>[4x]SRPVRLMKVFVTRRIPAEGRVALARAADCEVEQWDSDEPIPAKELERGVAGAHGLLCLLSDHVDKRILDAAGANLKVISTMSVGIDHLALDEIKKRGIRVGYTPDVLTDTTAELAVSLLLTTCRRLPEAIEEVKNGGWTSWKPLW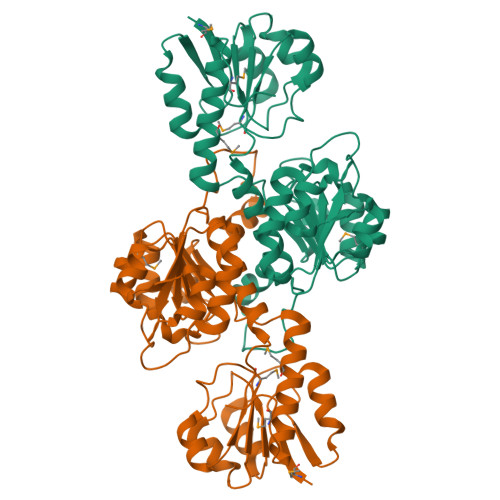LCGYGLTQSTVGIIGLGRIGQAIARRLKPFGVQRFLYTGRQPRPEEAAEFQAEFVSTPELAAQSDFIVVACSLTPATEGLCNKDFFQKMKETAVFINISRGDVVNQDDLYQALASGKIAAAGLDVTSPEPLPTNHPLLTLKNCVILPHIGSATHRTRNTMSLLAANNLLAGLRGEPMPSELKL>SYATKIHARYVYDSRGNPTVEVDFTTDKGLFRSIVPSGASTGVHEALELRDGDKSKWLGKGVLKAVANVNDIIAPALIKAKIDVVDQAKIDEFLLSLDGTPNKSKLGANAILGVSLAAANAAAAAQGIPLYKHIANISNAKKGKFVLPVPFQNVLNGGSHAGGALAFQEFMIAPTGVSTFSEALRIGSEVYHNLKSLTKKKYGQSAGNVGDEGGVAPDIKTPKEALDLIMDAIDKAGYKGKVGIAMDVASSEFYKDGKYDLDFKNPESDPSKWLSGPQLADLYEQLISEYPIVSIEDPFAEDDWDAWVHFFERVGDKIQIVGDDLTVTNPTRIKTAIEKKAANALLLKVNQIGTLTESIQAANDSYAAGWGVMVSHRSGETEDTFIADLSVGLRSGQIKTGAPARSERLAKLNQILRIEEELGSEAIYAGKDFQKASQL[4x]

The protein Eno1 (encoded by the ENO1 gene [C1_08500C_A]) plays a crucial role in the survival, pathogenicity, and antifungal drug susceptibilities of C. albicans. First, Eno1 has enolase activity and plays an essential role in glycolysis (catalyzing the conversion of 2-phospho-d-glycerate [2-PG] to phosphoenolpyruvate) in C. albicans, as knocking out the ENO1 gene renders C. albicans inviable on media with glucose as the sole carbon source. Second, Eno1 has transglutaminase activity and an ability to bind host plasminogen (PLG) and thus plays a key role in the invasion and virulence of C. albicans. Enolase is a dimeric enzyme and is critical for glycolysis, where it catalyzes the conversion of 2-PG to phosphoenolpyruvate.

The diffraction data show that in an asymmetric unit, four Eno1 proteins form two dimers. Two CaEno1 molecules form a homodimer face-to-face in an antiparallel manner. Interestingly the β4 to β13 strand forms a large β-barrel, while the α helices of the C-terminal domain are wrapped in the β-barrel to form a mixed α/β-barrel. This structure is similar to the three-dimensional structure of Eno1 in other species, suggesting that the active site of CaEno1 may also be in the C-terminal domain. The 2Fo-Fc electron density map of 2-PG and the key amino acid residues were contoured at 1.0 σ (gray) (right).>AGAGAMSIPSSQYGFVFNKQSGLKLRNDLPVHKPKAGQLLLKVDAVGLCHSDLAVIYEGLDCGDNYVMGHEIAGTVAAVGDDVINYKVGDRVACVGPNGCGGCKYCRGAIDNVCK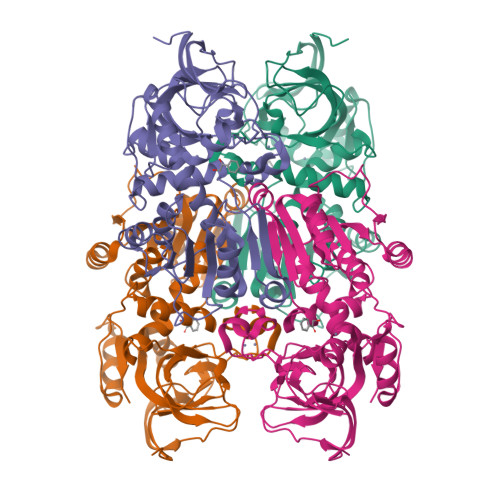NAFGDWFGLGYDGGYQQYLLVTRPRNLSRIPDNVSADVAAASTDAVLTPYHAIKMAQVSPTSNILLIGAGGLGGNAIQVAKAFGAKVTVLDKKKEARDQAKKLGADAVYETLPESISPGSFSACFDFVSVQATFDVCQKYVEPKGVIMPVGLGAPNLSFNLGDLALREIRILGSFWGTTNDLDDVLKLVSEGKVKPVVRSAKLKELPEYIEKLRNNAYEGRVVFNP[4x]>MNTVESRPVSVLFLCTGNTARSQLAQVLLEHHGGGRYAVTSAGLEPGS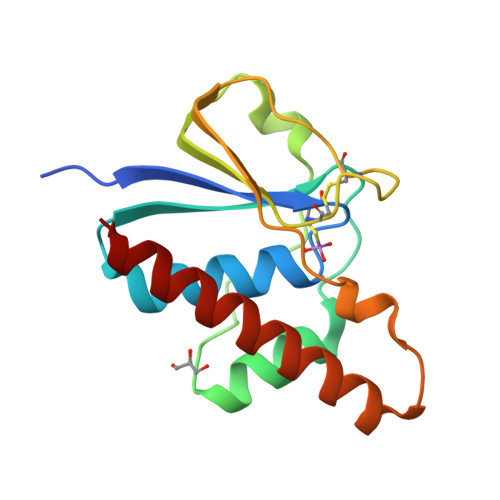VNPLTVQVLQESGLPTGHLQAKGVRPLIAEHFTYVITVCDRAEANCPIFPNATYRLHWPFEDPAAATGSEEERLAVFRHVRDEIDARIQAWVAARV[2x]2-deoxy-2-{[(2-hydroxy-1-methylhydrazino)carbonyl]amino}-beta-D-glucopyranose 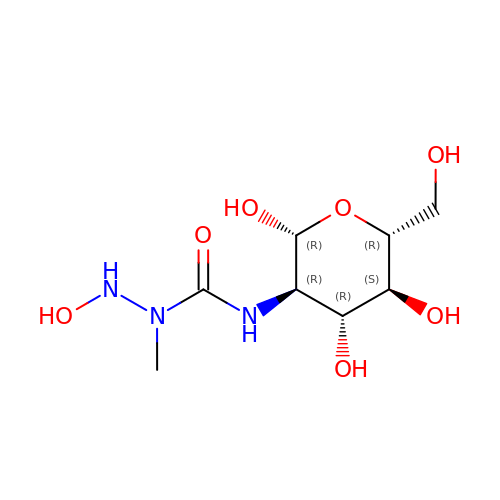| C8 H17 N3 O7 | LUNQAAUVSFIVKD-NYMZXIIRSA-N> PVFVPVPPPPLY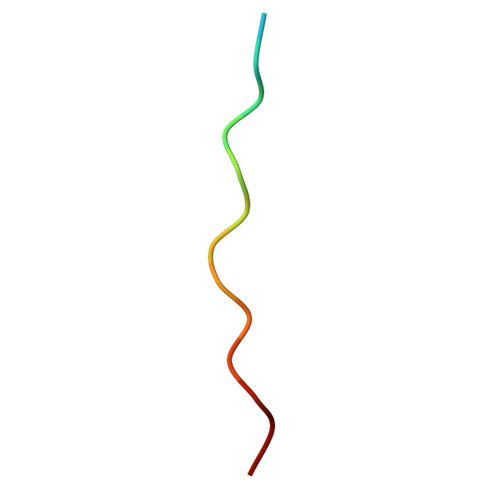PPP>[2x]GSVIDPSELTFVQEIGSGQFGLVHLGYWLNKDKVAIKTIREGAMSEEDFIEEAEVMMKLSHPKLVQLYGVCLEQAPICLVFEFMEHGCLSDYLRTQRGLFAAETLLGMCLDVCEGMAYLEEACVIHRDLAARNCLVGENQVIKVSDFGMTRFVLDDQYTSSTG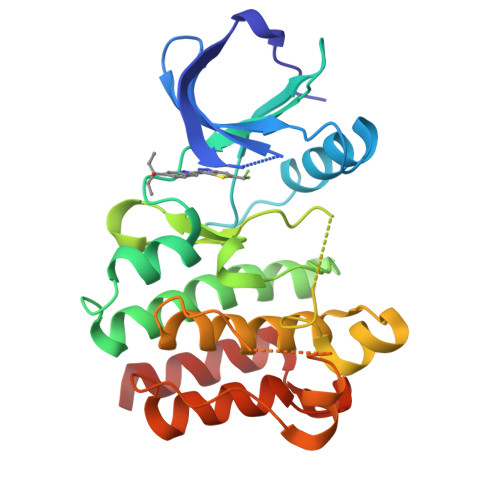TKFPVKWASPEVFSFSRYSSKSDVWSFGVLMWEVFSEGKIPYENRSNSEVVEDISTGFRLYKPRLASTHVYQIMNHCWKERPEDRPAFSRLLRQLAEIAESGL>GAMGIPQHQQKHALMAIKAVKRLKDARPFLQPVDPVALNIPLYFNFIKRPMDLQTIERKLNANAYE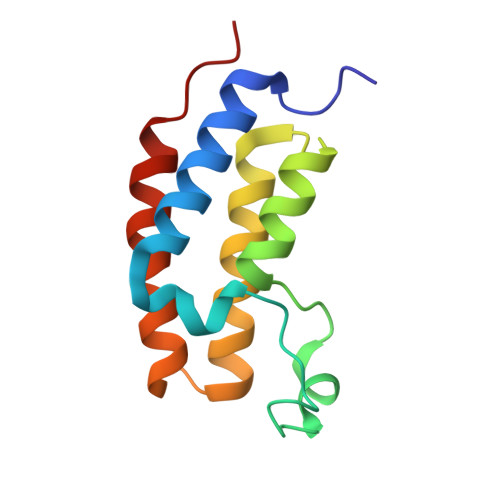TPEQITEDFNLMVENSAKFNGPTAVITQMGRNIQAAFEKHMLNMPAKD[2x]> APTAVEK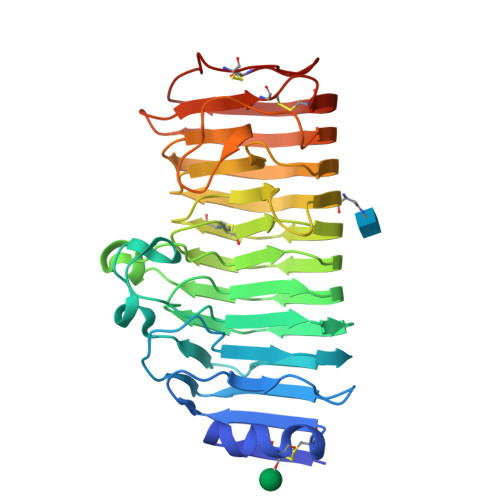RASCTFTDAASAMASKTACSTITLNNIAVPAGTTLDLTGLTSGTRVIFEGTTTFGYQEWSGPLVSISGTDITVQGASGSVLDGDGARWWDGQGSNGGKTKPKFFYAHSLDSSSITGITIKNSPVQVFSIQSNNLSLTDITVDDADGDTQGGHNTDAFDIGSSTYITITNANVHNQDDCIAVNSGENIIFTGGTCTGGHGLSIGSVGGRSDNTVKNVTIEHSTVTNSQNGVRIKTVYGATGSVSEVTYSNIQMSGIANYGIVIEQDYENGSPTGTPTNGVPITDLTLNTVTGSVSSGATEIYILCGSGSCSSWTWTGVSITGGSKSTKCENVPSGVSC> MSEYSQTVPELVSWARKNDFSISLPVERLAFLMAIAVLNSERLDGEMSEGELIDAFREVCKGFEQTAESVAVRANNAINDMVRQKLLNRFTSELADGNAIYRLTPLGISISDYYIRQREFSTLRLSMQLSIVANELHRAAEAAEEGGDEFHWHRNVFAPLKYSVAEIFDSIDMSQRLMDEQQNFVKEDIAALLNQDWQAAIANCEQLLSETSGTLRELQDTLEAAGDKLQANLLRIQDANMGSGGSELVDKLVFDLQSKLDRIIS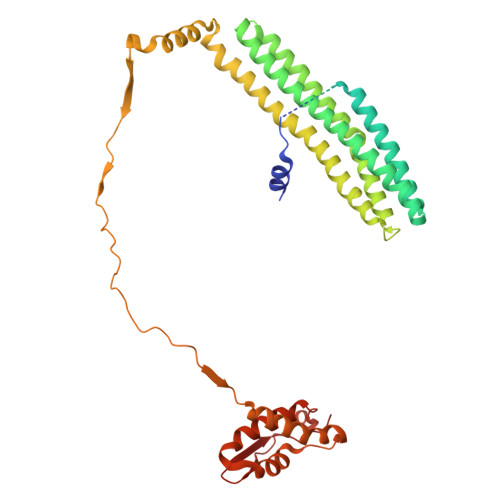WGQQAIDLWIGYDRHVHKFIRTAIDMDKNRIFSQRLRQSVQHYFDNPWTLTVANAERLLDMRDEELALRNEEVTGELPLELEYEEFSEINDQLAAMIEKALLVYQQEQRPLDLGAVLRDYLAQHPLPRHFDVARILVDQAVRLGVAEADFSGLPAEWLAINDYGAKVQAHVIDTY> MPIETKRQAEVLKKLQDVIKHTDRDIAAGRKLAIKRWVETYIEYIKLFKDDKLEFLYNVFRDEGCWLGTRLNNTVLGQKLTEEKIGEIDNPLPRYGMASRYCITGKIGDFFNKQFVLSRGQFTSEEVDSQGNPISDQYVRNILLSSMKRNGPVFDFWIDRESGELKKYDAVEGFDSTVKLKWSEGVEYFYNQLEEKDKEKKLTEAIVALSRPQSVKRDAPILDFCVRNIGDKDTLLQKLLQKDKGVYFLLAELIESCFFDTVHDLVQCWCYKGVSAGGDCSDKIFSQQDYELFLYSLSNVMLKNPELSVQARSLIMEIWKCERFAEYRETSVNTSNYTVPIKSVLGGLIINWKREDVCKPDREIEKEEILDMISFAKGCFPEKFDLFKEVMIENLRICGREGKRKGVDYGKFAEELFLQLEKVT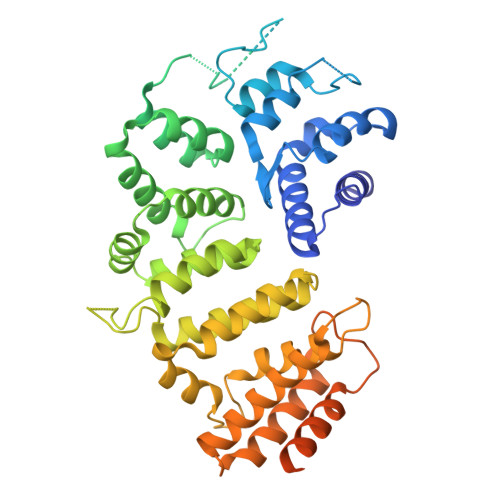LPSVGDGPWNNLRSQSKVSLPLDGSGDGPQSEFEAPSVSGISGSHKKRRILEHHHHHH> SAPGEDEECGRVRDFVAKLANNTHQHVFDDLRGSVSLSWVGDSTGVILVLTTFHVPLVIMTFGQSKLYRSEDYGKNFKDITDLINNTFIRTEFGMAIGPENSGKVVLTAEVSGGSRGGRIFRSSDFAKNFVQTDLPFHPLTQMMYSPQNSDYLLALSTENGLWVSKNFGGKWEEIHKAVCLAKWGSDNTIFFTTYANGSCKADLGALELWRTSDLGKSFKTIGVKIYSFGLGGRFLFASVMADKDTTRRIHVSTDQGDTWSMAQLPSVGQEQFYSILAANDDMVFMHVDEPGDTGFGTIFTSDDRGIVYSKSLDRHLYTTTGGETDFT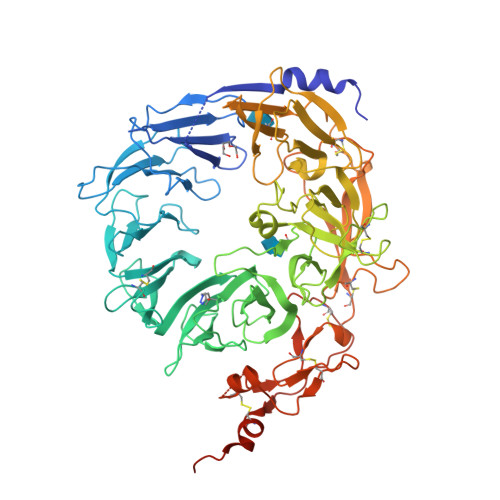NVTSLRGVYITSVLSEDNSIQTMITFDQGGRWTHLRKPENSECDATAKNKNECSLHIHASYSISQKLNVPMAPLSEPNAVGIVIAHGSVGDAISVMVPDVYISDDGGYSWTKMLEGPHYYTILDSGGIIVAIEHSSRPINVIKFSTDEGQCWQTYTFTRDPIYFTGLASEPGARSMNISIWGFTESFLTSQWVSYTIDFKDILERNCEEKDYTIWLAHSTDPEDYEDGCILGYKEQFLRLRKSSMCQNGRDYVVTKQPSICLCSLEDFLCDFGYYRPENDSKCVEQPELKGHDLEFCLYGREEHLTTNGYRKIPGDKCQGGVNPVREVKDLKKKCTSNFLSPEKQNSKSNSGSAMIEGRGVGHHHHHH>EAEAADRADILYNIRQTSRPDVIPTQRDRPVAVSVSLKFINILEVNEITNEVDVVFWQQTTWSDRTLAWDSSHSPDQVSVPISSLWVPDLAAYNAISKPEVLTPQLARVVSDGEVLYMPSIRQRFSC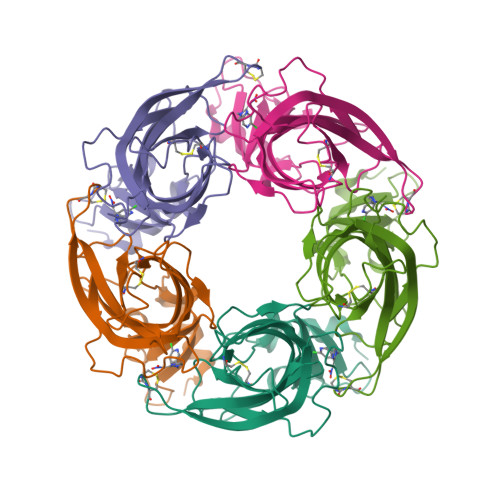DVSGVDTESGATCRIKIGSWTHHSREISVDPTTENSDDSEYFSQYSRFEILDVTQKKNSVTYSCCPEAYEDVEVSLNFRKKGRSEIL[5x]> MSGSNSTANGANSTASGDNSTASGTNASATGENSTATGTDSTASGSNSTANGTNSTASGNNSTASGTNASATGENSTATGTDSAASGTNSTANGTNSTASGDNSTASGTNASATGENSTATGTASTASGSNSTANGANSTASGAGATATGENAAATGAGATATGNNASASGTSSTAGGANAIASGENSTTNGANSTASGNGSSAFGESAAAAGDGSTALGANAVASGVGSVATGAGSVASGANSSAYGTGSNATGAGSVAIGQGATASGSNSVALGTGSVASEDNTVSVGSAGSERRITNVAAGVNATDAVNVGQMKQIEDKIEEILSKIYXXXXXXXXXXXXXXXXXXXX

Gram‐negative pathogens like Burkholderia pseudomallei use trimeric autotransporter adhesins such as BpaC as key molecules in their pathogenicity. The TAA BpaC was first extensively described in 2013 (Campos et al., 2013); of the nine predicted B. pseudomallei TAAs, BpaC is the only one associated with all of the three features involved in pathogenicity: macrophage survival, virulence, and serum survival (Lazar Adler et al., 2015). Studies have demonstrated BpaC adhesion to respiratory epithelial cell lines, establishing the importance of BpaC in the initial attachment and tropism of the pathogen (Lafontaine et al., 2014).

Our 1.4 Å crystal structure of the membrane‐proximal part of the BpaC head domain shows that the domain is exclusively made of left‐handed parallel β‐roll repeats. Having settled on BpaC741–1054 as the region to express, we used the engineered trimeric GCN4 leucine zipper (Hernandez Alvarez et al., 2008) to preserve the DAVNxxQL neck motif at the C‐terminal end by replacing the coiled‐coil that would be in the membrane β‐barrel in the wt structure. There was a single molecule in the asymmetric unit, and the TAA trimer formed around the crystallographic threefold axis. The final model contains all of the residues in BpaC from position 14 in layer 22 to the end of layer 42 (residues 741–1021), followed by a long neck from E1022 to Q1054, the GCN4 anchor, with 282 water molecules, of which 42 are ordered in specific channels or the trimer core cavity. All three chains of the C‐terminal head domain of BpaC thread around a central hydrophilic core in a helical fashion with an average turn of 5.7° ± 0.6° for layers 23–41 and a rise of 4.8 Å ± 0.1 Å (the last one, from 1008–1021, has a turn of just 2.5°), calculated per turn, typical of other LPBRs. Instead of predominantly β‐branched hydrophobic residues (Nummelin et al., 2004) at positions 5 and 7, BpaC has T@5 almost exclusively as well as a number of hydrophilic residues with T/N/S/G@7. More surprising, however, are the “inner” and “central” chains of buried water molecules, which form because the BpaC core is uniquely hydrophilic in 15/20 of the LPBR layers, composed of repeating units of N/S/T@7. In BpaC, only negatively charged residues face the solvent—in stark contrast to the primarily positive surface charge of the left‐handed parallel β‐roll “type” protein, YadA. The pIs of the solved LPBR structures demonstrate this clearly: the pI of the LPBR is clearly correlated with its position within the passenger domain, with BpaC having a pI of about 2.3 and YadA of 9.2. The structure reported here of BpaC741–1054 contains the highest number of LPBR repeats in an experimental structure and is the longest, at 89.5 Å.> MSQNQVPKWIQLNNEIMIQKDGKFQFDKDKEAVHSYFVDYINQNTVFFHNLKEKLDYLVENQYYEEEFLSLYSFEDIKEVFKTAYAKKFRFPSFMSAFKFYNDYALKTNDKKKILERYEDRISIVALFFANGDTEKAKEYVNLMINQEYQPSTPTFLNAGRKRRGELVSCFLLEVNDSLNDISRAIDISMQLSKLGGGVSLNLSKLRAKGEAIKDVENATKGVVGVMKLLDNAFRYADQMGQRQGSGAAYLNIFHRDINDFLDTKKISADEDVRVKTLSIGVVIPDKFVELAREDKAAYVFYPHTIYKEYGQHMDEMDMNEMYDKFVDNPRVKKEKINPRKLLEKLAML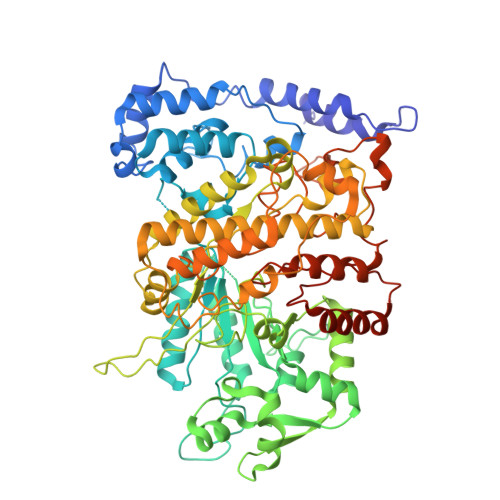RSESGYPYIMFQDNVNKVHANNHISKVKFSNLCSEVLQASQVSSYTDYDEEDEIGLDISCNLGSLNILNVMEHKSIEKTVKLATDSLTHVSETTDIRNAPAVRRANKAMKSIGLGAMNLHGYLAQNGIAYESPEARDFANTFFMMVNFYSIQRSAEIAKEKGETFDQYEGSTYATGEYFDKYVSTDFSPKYEKIANLFEGMHIPTTEDWKKLKAFVAEHGMYHSYRLCIAPTGSISYVQSSTASVMPIMERIEERTYGNSKTYYPMPGLASNNWFFYKEAYDMDMFKVVDMIATIQQHIDQGISFTLFLKDTMTTRDLNRIDLYAHHRGIKTIYYARTKDTGQDSCLSCVV>MGSHHHHHHENLYFQGHMNSFYSQEELKKIGFLSVGKNVLISKKASIYNPGVISIGNNVRIDDFCILSGKVTIGSYSHIAAYTALYGGEVGIEMYDFANITSRTIVYAAIDDFSGNALMGPTIPNQYKNVKTGKVILKKHVIIGAHSIIFP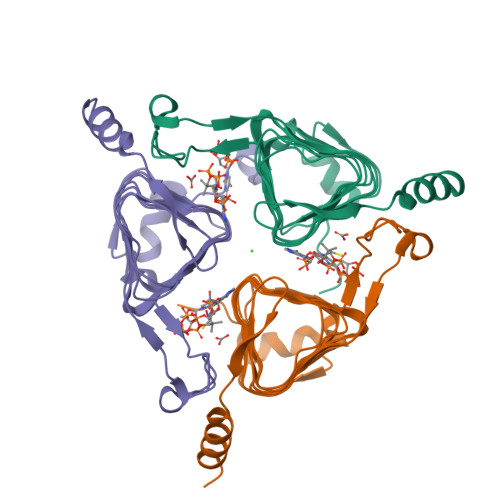NVVIGEGVAVGAMSMVKESLDDWYIYVGVPVRKIKARKRKIVELENEFLKSMNS[3x]> GQPEYPVIRLNDELEVREILPNAFVITHKFPWGGNSLVVLIGEKYAVFVDTPYTPEATENVLDWINKQYGNRQFIEINTGYHVDNLGGNDALLHRNIPIIGSDKTVSLLRERGEATRQLTMGWLEGPGNEKFLKRHETIPYVGPSQIFQLTEG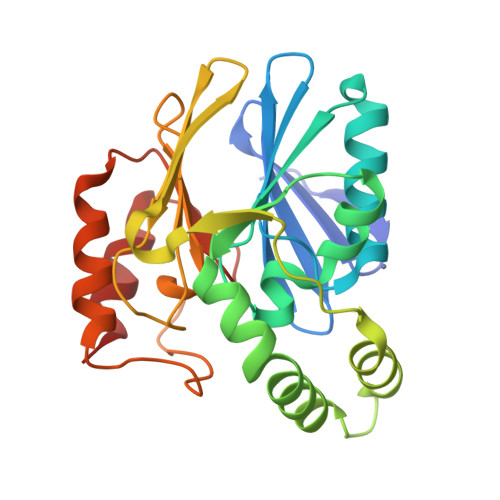YHFTVGDEPIEVFFPGETHAPDNIVVYFPERKILFGGCMLRVGNGTGNRADANMDTWKSSVERLRDFDCVAVIPGHGIRFDPGVIENTISVLP> MSSIPWIDNEFAYRALAHLPKFTQVNNSSTFKLRFRCPVCGDSKTDQNKARGWYYGDNNEGNIHCYNCNYHAPIGIYLKEFEPDLYREYIFEIRKEKGKSRPIEKPKELPKQPEKKIIKSLPSCVRLDKLAEDHPIIKYVKARCIPKDKWKYLWFTTEWPKLVNSIAPGTYKKEISEPRLVIPIYNANGKAESFQGRALKKDAPQKYITIEAYPEATKIYGVERVKDGDVYVLEGPIDSLFIENGIAITGGQLDLEVVPFKDRRVWVLDNEPRHPDTIKRMTKLVDAGERVMFWDKSPWKSKDVNDMIRKEGATPEQIMEYMKNNIAQGLMAKMRLSKYAKI

The T4 bacteriophage gp41 helicase and gp61 primase assemble into a primosome to couple DNA unwinding with RNA primer synthesis for DNA replication. The domain architecture of the gp41 helicase resembles the bacterial DnaB helicase13,14 with an NTD and a RecA-like CTD that are connected by a linking helix (LH). The gp61 primase is composed of an N-terminal ZBD and a C-terminal RPD that are linked by an 18-residue flexible loop. Here we report a series of cryo-EM structures of T4 primosome assembly intermediates.

Therefore, we utilized an inactive gp41 helicase mutant with an E227Q substitution in the walker-B motif that abolished the ATP-hydrolysis activity, and assembled a T4 primosome with the WT gp61 primase and the ssDNA/RNA primer substrate. We separately refined the helicase and primase regions to improve the resolution. The gp61 primase region achieved ~4.0 Å local resolution where the pentaribonucleotide primer was observed to form a short hybrid duplex with the template DNA that was absent in the WT primosome map. The RNA primer density was just enough to accommodate five ribonucleotides, consistent with the RNA primer provided. The 5-nt RNA primer extends from the gp61 ZBD to the NTL of the gp61 RPD. The primer 5’-triphosphate group is stabilized by Arg51 in the gp61 ZBD loop region; similar to the interaction observed in the T7 gp4 ZBD–ssDNA/RNA primer structure. In the gp61 RPD, the RNA primer binds to the NTL and displaces the ssDNA bound there in the WT primosome structure. The 3’-end of the primer is stabilized by the β-hairpin of the gp61 RPD. Interestingly, the 3′-OH of the primer has passed over the catalytic site in the mutant structure, such that no additional ribonucleotides can be added in this configuration. Indeed, we found that the linker loop stretched and became ordered in the mutant T4 primosome bound to a completed 5-nt RNA primer, as compared to the disordered linker loop in the ssDNA template-bound WT primosome.> MGHHHHHHHHHHEPPAIPHITEGFYPLPEIVETFSHHVLQELVSLAEVLPSMSNVEKKKKILDWLLRSRAFTMRLLVLARWVHLSPSVHRCIDVVAFLQGQKFCF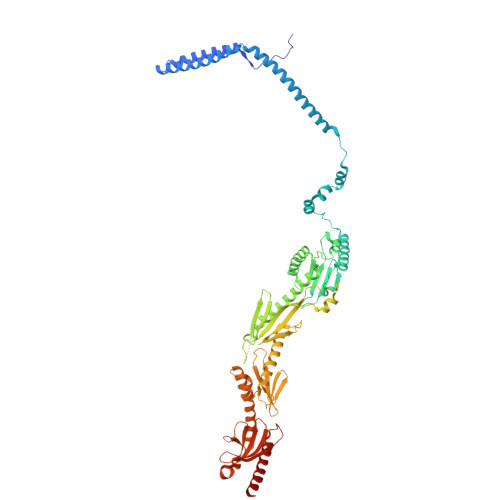QNLVHVLQDIRYQLSFARLRNSDLVTALDILSTGTSLRLANAPTSKLYMLSESPLSTKQILQTLHALNMLIRIRLSLYEIIPTPFQHFTIANGRCTFTVPNEFSVSLTTNSQDPKSTGISFQWIVVDFQFHLPDFSSTPAKYRVFIELHLNEEIAAAFVLQKPILPLIYNILHKFCLYQRLNLLSQQTFQLSRESWLGHLRGVYDEKPPRLRLYYWPQLNVKKEGKPGKIGHYIHIFVNTQPISAFERTLSSKRSSCEYDHFLLLVEWHHDGIVEHVPLDDHMDAQHLLLLITQKHAQLILEQIRKELHPNIFSEHVGGGLKIHVFDNEIIVKVNSVTGRLVLSSSASPLSPPRHLRAAEKNIALNTQPPAQILNRLYFFCIQTQLLEVAQCAELHAVQGYYSFPYLTFSKGKWRKDGDSLWVLAYNVESNSWSVRLLNAAGQTLYTQDVHTTKGTLSIESFSRLSYLLEVQILLFNVQTACQARG> MAIYADNSYSIGNTPLVRLKHFGHNGNVVVKIEGRNPSYSVKCRIGANMVWQAEKDGTLTKGKEIVEPTSG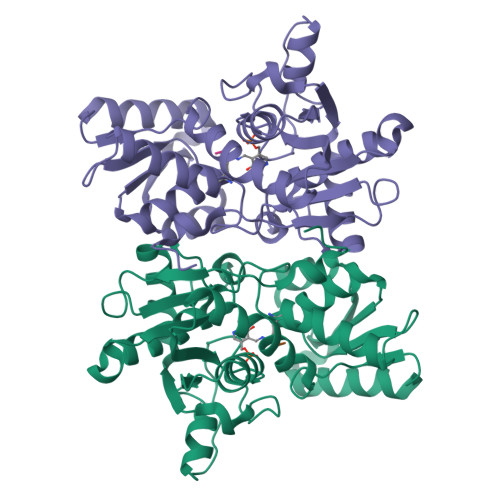NTGIALAYVAAARGYKITLTMPETMSIERKRLLCGLGVNLVLTEGAKGMKGAIAKAEEIVASDPSRYVMLKQFENPANPQIHRETTGPEIWKDTDGKVDVVVAGVGTGGSITGISRAIKLDFGKQITSVAVEPVESPVISQTLAGEEVKPGPHKIQGIGAGFIPKNLDLSIIDRVETVDSDTALATARRLMAEEGILAGISSGAAVAAADRLAKLPEFADKLIVVILPSSSERYLSTALFEGIEG;> DGMNLNI1-[(6-aminopyridin-3-yl)methyl]-3-[4-(phenylsulfonyl)phenyl]urea | C19 H18 N4 O3 S 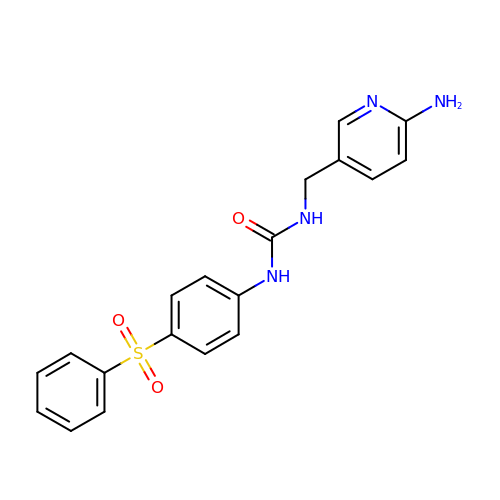| CYPHXCMPISHSDL-UHFFFAOYSA-N>[2x]MNDMRQITNLGRNIENKSFSIIDEEAGPHSF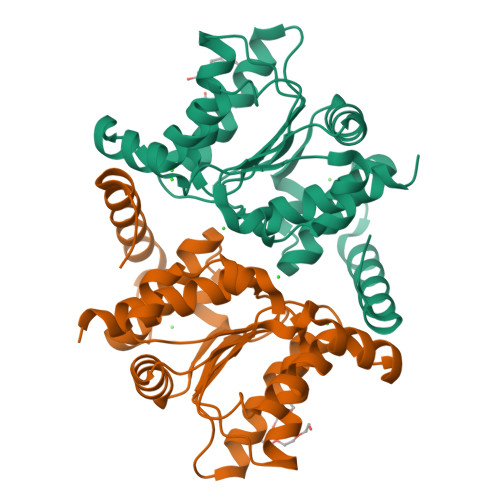AQEEWEVVRRIIHATADFDYKNITKIHPQAIDSGIQALKKGCPIVCDVQMILSGLNPERLKVYGCKTYCFISDEDVIENAKRKNSTRAIESIQKANSFNLLNESIIVIGNAPTALLEIEKLIRQEGIKPALIVGVPVGFVSAKESKESILKLEYYNVTSIPYILTMGRKGGSTIAVAILHALLLLSSKRGERLEHHHHHH>[6x]SNAMTQEQQLSGGELSLPNGELVLRTLAMPADTNANGDIFGGWLMSQMDIGGAIQAKEIAQGRVVTVRVDGMTFLKPVAVGDVVCCYARCIKTGHSSITINIEVWVK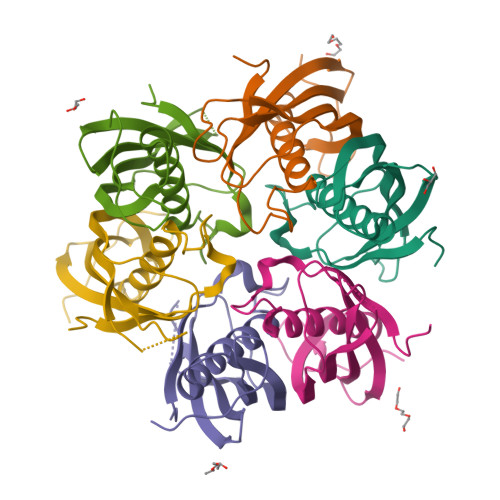KVSSEPIGQRYRATEAVFTYVAVDDAGKPRGLPSGKGNFEVGATQ>[2x]MEFFGETWRRELAAEFEKP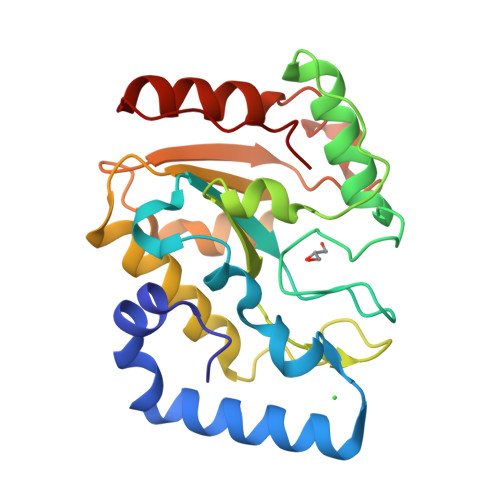YFKQLMSFVADERSRHTVYPPADQVYSWTEMCDIQDVKVVILGQDPYHGPNQAHGLCFSVQKPVPPPPSLVNIYKELCTDIDGFKHPGHGDLSGWAKQGVLLLNAVLTVRAHQANSHKDRGWETFTDAVIKWLSVNREGVVFLLWGSYAHKKGATIDRKRHHVLQAVHPSPLSAHRGFLGCKHFSKANGLLKLSGTEPINWRAL> MASEAKQTVHTGNTVLLMIKGKPVGRAQSASGQREYGTTGVYEIGSIMPQEHVYLRYEGTITVERLRMKKENFADLGY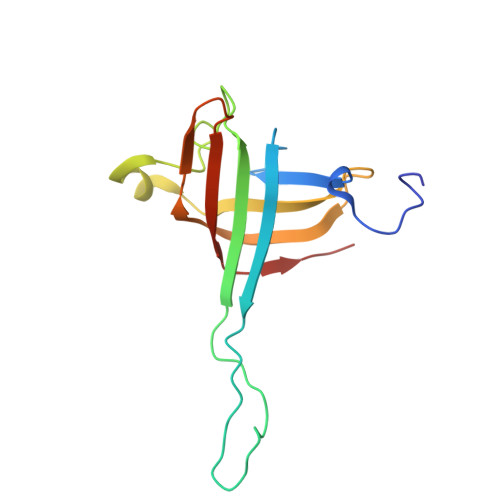ASLGEEILKKDIIDILVVDNLTKQVIISYHGCSANNYNETWQTNEIVTEEIEFSYLTASDKART>[2x]MALNGAEVDDFSWEPPTE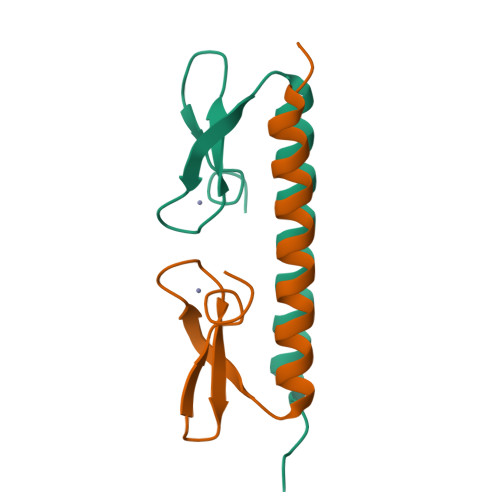AETKVLQARRERQDRISRLMGDYLLRGYRMLGETCADCGTILLQDKQRKIYCVACQELDSDVDKDNPALNAQAALSQAREHQLASASELPLGSRPAPQPPVPRPEHCEGAAAGLKAAQGPPAPAVPPNTDVMACTQTALLQKLTWASAELGSSTSLETSIQLCGLIRACAEALRSLQQLQH>[2x]MAEKRNIFLVGPMGAGKSTIGRQLAQQ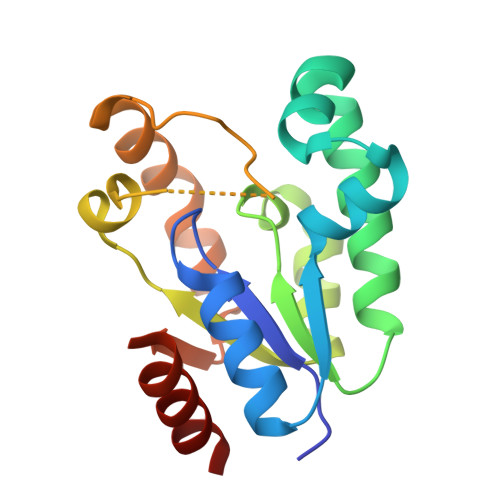LNMEFYDSDQEIEKRTGADVGWVFDLEGEEGFRDREEKVINELTEKQGIVLATGGGSVKSRETRNRLSARGVVVYLETTIEKQLARTQRDKKRPLLHVETPPREVLEALANERNPLYEEIADVTIRTDDQSAKVVANQIIHMLESN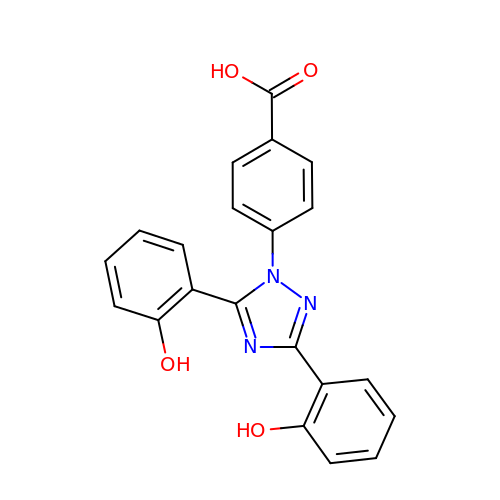4-[3,5-bis(2-hydroxyphenyl)-1,2,4-triazol-1-yl]benzoic acid | C21 H15 N3 O4 | BOFQWVMAQOTZIW-UHFFFAOYSA-N>METESGNQEKVMEEESTEKKKEVEKKKRSRVKQVLADIAKQVDFWFGDANLHKDRFLREQIEKSRDGYVDISLLVSFNKMKKLTTDGKLIARALRSSAVVELDLEGTRIRRKKPLGERPKDEDERTVYVELLPKNVNHSWIERVFGKCGNVVYISIPHYKSTGDPKGFAFVEFETKEQAAKAIEFLNNPPEEA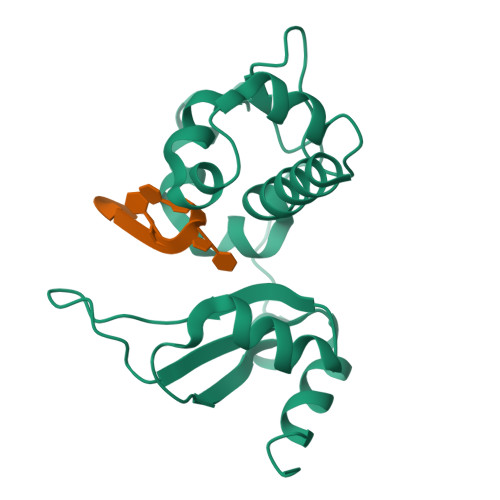PRKPGIFPKTVKNKP[2x]> MVDMSKVKLRIENIVASVDLFAQLDLEKVLDLCPNSKYNPEEFPGIICHLDDPKVALLIFSSGKLVVTGAKSVQDIERAVAKLAQKLKSIGVKFKRAPQIDVQNMVFSGDIGREFN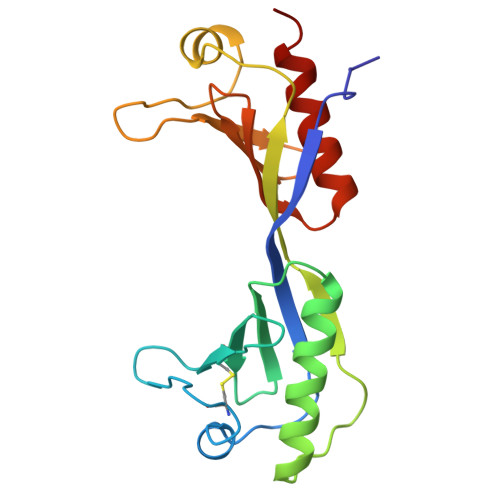LDVVALTLPNCEYEPEQFPGVIYRVKEPKSVILLFSSGKIVCSGAKSEADAWEAVRKLLRELDKYL>[4x]GSKNYIEMKPHPWFFGKIPRAKAEEMLSKQRHDGAFLIRESESAPGDFSLSVKFGNDVQHFKVLRDGAGKYFLWVVKFNSLNEL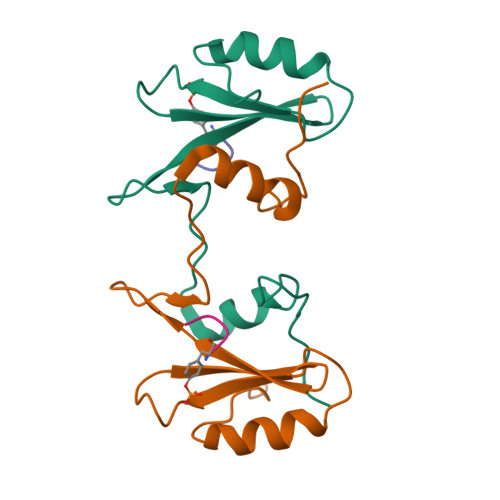VDYHRSTSVSRNQQIFLRDIEQVPQQPTYV;>XYVNV[4x]>GPVSVANHLGEDAGHLALRRDVYSGLQKTPKSLPPKWFYDTVGSELFDQITRLPEYYPTRAEAEILRARSAEVASACRADTLVELGSGTSEKTRMLLDALRHRGSLRRFVPFDVDASVLSATATAIQREYSGVEINAVCGDFEEHLTEIPRGGRRLFVFLGSTIGNLTPGPRAQFLTALAGVMRPGDSLLLGTDLVKDAARLVRAYDDPGGVTAQFNRNVLAVINRELEADFDVDAFQHVARWNSAEERIEMWLRADGRQRVRVGALDLTVDFDAGEEMLTEVSCKFRPQAVGAELAAAGLHRIRWWTDEAGDFGLSLAAK[2x]

EgtD, an S-adenosylmethionine-dependent methyltransferase (AdoMet), catalyzes the trimethylation of L-Histidine to initiate EGT biosynthesis and this reaction has been shown to be essential for EGT production in mycobacteria and for long-term infection of murine macrophages by M. tb. Synthesis of EGT by Mycobacterium tuberculosis (M. tb) is critical for maintaining bioenergetic homeostasis and protecting the bacterium from alkylating agents, oxidative stress, and anti-tubercular drugs. Multiple X-ray crystal structures of Mycolicibacterium smegmatis EgtD show that EgtD possesses a Histidine binding domain and a Rossmann-fold domain, which affords ordered substrate binding of L-Histidine and AdoMet, respectively. In this work, library screening and structure-guided strategies identified multiple classes of M. tb EgtD inhibitors that bind in various regions of the enzyme active site.

The two rings of Imatinib modeled within the L-Histidine binding pocket are well-resolved. The remainder of Imatinib extends to the AdoMet binding site resulting in a lack of difference density representing those three heterocycles. The pyridine ring sits within the imidazole binding subsite and forms π-π interactions with Tyr206 and eleven close (shorter than 4.0 Å) van der Waals interactions with the surrounding hydrophobic residues. In addition, the nitrogen atom of the pyridine ring forms a hydrogen bond with the ordered water molecule analogous to the imidazole-water interaction observed in the L-Histidine derivative structures. The pyrimidine ring forms only three van der Waals interactions and three hydrogen bonded interactions with two ordered water molecules and the side chain of Thr163. The pyridine-pyrimidine rings of Imatinib are positioned in the histidine binding pocket by an extensive network of interactions. Superimposing the Imatinib complex with the M. smegmatis EgtD-L-Histidine complex illustrates distinct modes of binding site engagement. Where L-Histidine interacts with EgtD primarily through polar interactions, Imatinib interacts through almost exclusively van der Waals interactions. Based on these results, it is intriguing to consider that M. tb EgtD is a biological target for Imatinib and that inhibition of EGT production during an infection is the reason for the observed drug synergy.> MHHHHHHMDYLPERDVYESLCRGEGVKLTPRRQKRLFCRYHHGNRAPQLLIAPFKEEDEWDSPHIVRYYDVMSDEEIERIKEIAKPKLARATVRDPKTGVLTVASYRVSKSSWLEEDDDPVVARVNR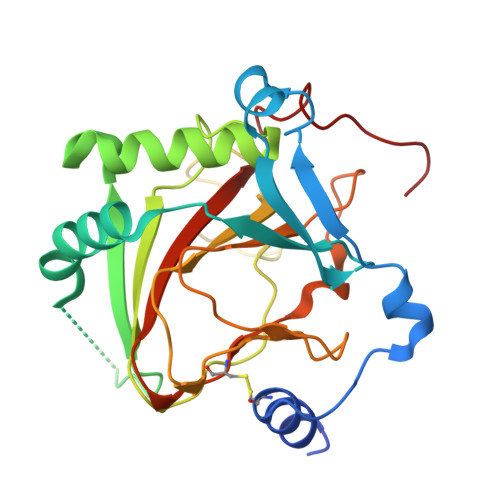RMQHITGLTVKTAELLQVANYGVGGQYEPHFDFSRNDERDTFKHLGTGNRVATFLNYMSDVEAGGATVFPDLGAAIWPKKGTAVFWYNLLRSGEGDYRTRHAACPVLVGCKWVSNKWFHERGQEFLRPCGSTEVD> S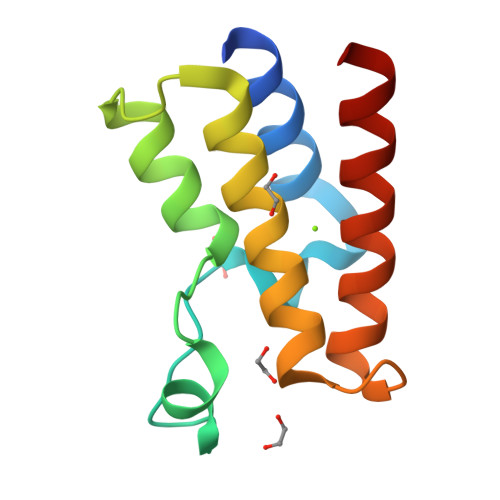MHSDLTFCEIILMEMESHDAAWPFLEPVNPRLVSGYRRIIKNPMDFSTMRERLLRGGYTSSEEFAADALLVFDNCQTFNEDDSEVGKAGHIMRRFFESRWEEFYQ> KVEQAVETEPEPELRQQTEWQSGQRWELALGRFWDYLRWVQTLSEQVQEELLSSQVTQELRALMDETMKELKAYKSELEEQLTPVAEETRARLSKELQAAQARLGADMEDVCGRLVQYRGEVQAMLGQSTEELRVRLASHLRKLRKRLLRDADALQKCLAVYQA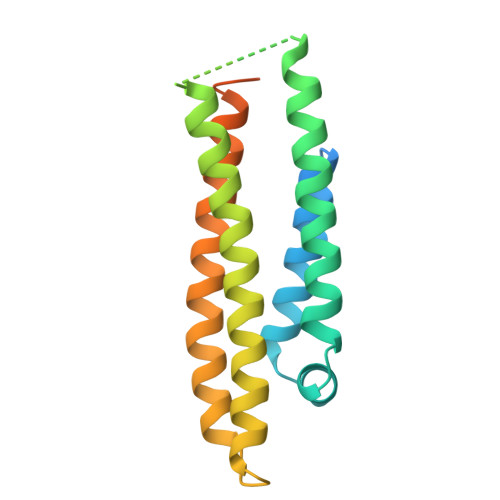GAREGAERGLSAIRERLGPLVEQGRVR>[10x]APADNAADARPVDVSVSIFINKIYGVNTLEQTYKVDGYIVAQWTGKPRKTPGDKPLIVENTQIERWINNGLWVPALEFINVVGSPDTGNKRLMLFPDGRVIYNARFLGSFSNDMDFRLFPFDRQQFVLELEPFSYNNQQLRFSDIQVYTENIDNEEIDEWWIRGKASTHISDIRYDHLS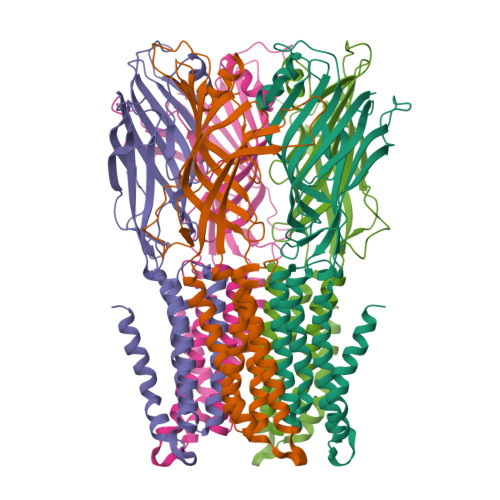SVQPNQNEFSRITVRIDAVRNPSYYLWSFILPLGLIIAASWSVFWLESFSERLQTSFTLMLTVVAYAFYTSNILGRLPYTTVIDQMIIAGYGSIFAAILLIIFAHHRQANGVEDDLLIQRCRLAFPLGFLAIGCVLVIRGITL>[5x]MLSAFQLENNRLTRLEVEESQPLVNAVWIDLVEPDDDERLRVQSELGQSLATRPELEDIEASARFFEDDDGLHIHSFFFFEDAEDHAGNSTVAFTIRDGRLFTLRERELPAFRLYRMRARSQSMVDGNAYELLLDLFETKIE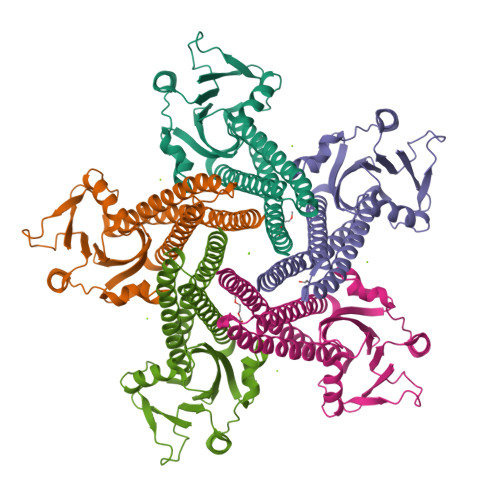QLADEIENIYSDLEQLSRVIMEGHQGDEYDEALSTLAELEDIGWKVRLCLMDTQRALNFLVRKARLPGGQLEQAREILRDIESLLPHNESLFQKVNFLMQAAMGFINIEQNRIIK>MSGSHHHHHHSGSMSERPSDLVVNRLVLFVVKGTATSTHDTVKPLILLEELGVPHDIYVVEKVSAPWFSEINPHKMVPAILDRSPDGRDTLRAWESTSTLMYIADAYDKDGTFGGRNVQERSEINNWLTLHTAALGPTAKYWLYFYKLHPEKLPKTI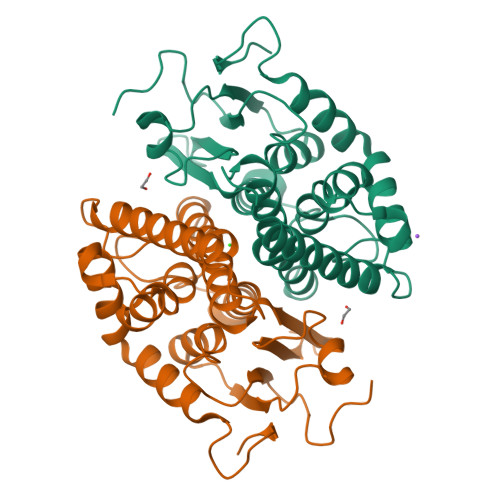EKLRSNITVQYDILERRLNEPGQQYLALKDRPTIADIATLPFAMKSTAELFGLEFEKWPKLQEWSVRMGEREAVKRAWQRVAGFGHGEKEYGMLEA[6x]>MELGAGGVVFNAKREVLLLRDRMGFWVFPKGHPEPGESLEEAAVREVWEETGVRAEVLLPLYPTR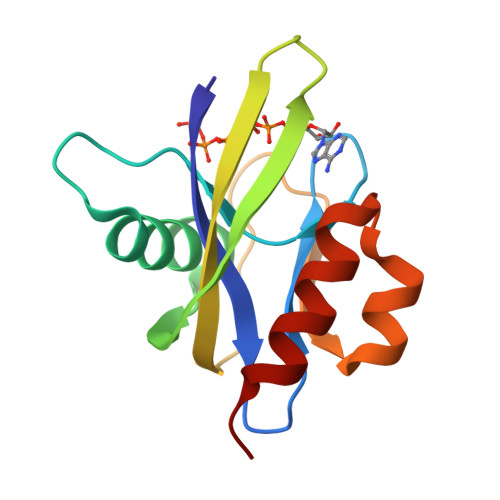YVNPKGVEREVHWFLMRGEGAPRLEEGMTGAGWFSPEEARALLAFPEDLGLLEVALERLPL[2x]>[2x]AFKEDNTVAFKHLFLKGYSGTDEDDYSCSVYTQ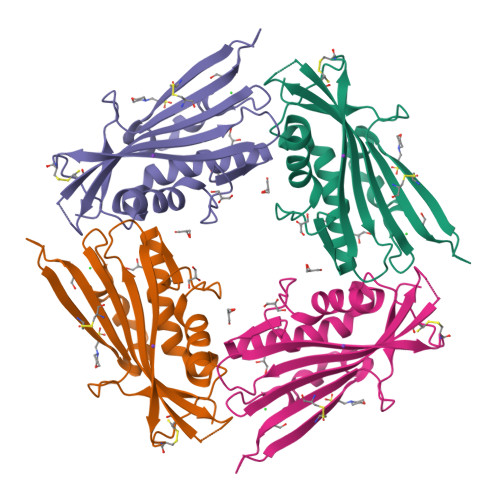EDAYESIFFAINQYHQLKDITLGTLGYGENEDNRIGLKVCKQHYKKGTMFPSNETLNIDNDVELDCVQLDLQDLSKKPPDWKNSSFFRLEFYRLLQVEISFHLKGIDLQTIHSRELPDCYVFQNTIIFDNKAHSGKIKIYFDSDAKIEECKDLNIFGS A trait of BP bacteria is a conserved gene cluster coding for the biosynthesis of polyketides (malleicyprols) with a reactive cyclopropanol unit that is critical for virulence. We show that BurG, an unusual NAD+-dependent member of the ketol-acid reductoisomerase family, constructs the strained cyclopropanol ring. A sequence similarity search using BLAST predicted that BurG belongs to the family of ketol-acid reductoisomerases (KARIs; EC 1.1.1.86), well-characterized enzymes that play key roles in the biosynthesis of branched-chain amino acids. Biochemical assays and a suite of eight crystal structures of native and mutated BurG with bound analogues and inhibitors provide snapshots of each step of the complex reaction mechanism, involving a concealed oxidoreduction and a C–S bond cleavage.

Apart from its function as a catalytic base, E232 also plays an active role in substrate recognition and positioning as we gleaned from crystallization assays with gonydiol and BurG. In one subset the active centre is populated by the enzymatic reaction products 6 and DMS. The second subset clearly depicts the backbone of gonydiol, which was oxidized into its enolate 14. Intermediate 14 is firmly held in place by ionic interaction of its sulfonium moiety with E232 and cation–π interaction with Y133. In addition, the glutamate residue (E232) would ionically interact with the positively charged sulfonium group to firmly position the substrate in the binding pocket. Inheritance of the redox capability of KARIs allows BurG to activate its substrate gonydiol as the electrophilic intermediate 14. This activation is vital for intramolecular electrophilic displacement of DMS as leaving group and subsequent cyclopropanol formation. In the case of BurG, formation of 6 is probably driven by a gain in entropy and removal of the volatile DMS from the chemical equilibrium after cyclopropanol synthesis.

>[2x]GSHMASNDLIYQDEHASLQPLEGRTVAVIGYGIQGRAFAANLRDSGVAVRVGNIDDRYFELARAEGHRVTNIAEAVAHADIVLLLIPDEAHGAVFDVDIAPNLRDGALLCVAHGHSLVQGDVRPLPGRDLAMLAPRMYGDPIRRYYLAGQGAPAYFDIVADHTGRARDRVLAIARAVGFTRAGVMALGYRQETFLDLFQEQFLAPALVDLVETGFQVLVERGFNPKAALLEVYGSGEMGKMMLDGADIGLDEVVALQGSPTCQVGYHRWRGRTLPTAVRELAARVLDQIEGGDFSAYLKEQASNDYASLDDARRAALKRPLNVAHAQVRAAFRFPTEAAGGLYQAAQAPADVEPEAAR> SDVDLSKYITTIAGVMTLSQVKGFVRKNGVNEAKIDEIKNDNVQDTAEQKVQLLRNWHQLHGKKEAYDTLIKDLKKA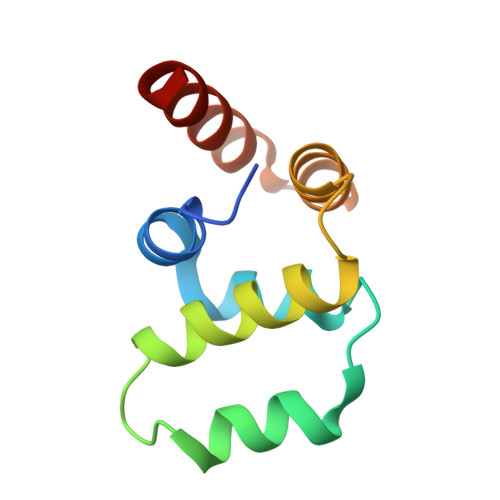NLCTLAEKIQTIILKDITS>[2x]MGSSHHHHHHHSQDPAEKQKHDGRVKIGHYVLGDTLGVGTFGKVKIGEHQLTGHKVAVKILNRQKIRSLDVVGKIKREIQNLKLFRHPHIIKLYQVISTPTDFFMVMEYVSGGELFDYICKHGRVEEMEARRLFQQILSAVDYCHRHMVVHRDLKPENVLLDAHMNAKIADFGLSNMMSDGEFLRTSCGSPNYAAPEVISGRLYAGPEVDIWSCGVILYALLCGTLPFDDEHVPTLFKKIRGGVFYIPEYLNRSVATLLMHMLQVDPLKRATIKDIREHEWFKQDLPSYLFPEDPSYDANVIDDEAVKEVCEKFECTESEVMNSLYSGDPQDQLAVAYHLIIDNRRIMNQASEFYLASSPPDSFLDDHHLTRPHPERVPFLVAETPRARHTLDELNPQKSKHQGVKKAKWHLGIRSQSKPYDIMAEVYRAMKQLDFEWKVVNAYHLRVRRKNPVTGNYVKMSLQLYLVDNRSYLLDFKSIDDEVVEQRSGSSTPQRSCSAAGLHRPRSSFDSTTAESHSLSGSLTGSLTGSTLSSVSPRLGSHTMDFFEMCASLITTLAR;>MGNTSSERAALERHGGHKTPRRDSSGGTKDGDRPKILMDSPEDADLFHSEEIKAPEKEEFLAWQHDLEVNDKAPAQARPTVFRWTGGGKEVYLSGSFNNWSKLPLTRSHNNFVAILDLPEGEHQYKFFVDGQWTHDPSEPIVTSQLGTVNNIIQVKKTDFEVFDALMVDSQKCSDVSELSSSPPGPYHQEPYVCKPEERFRAPPILPPHLLQVILNKDTGISCDPALLPEPNHVMLNHLYALSIKDGVMVLSATHRYKKKYVTTLLYKPI[2x];>MADLNWETVISSDSSPAVENEHPQETP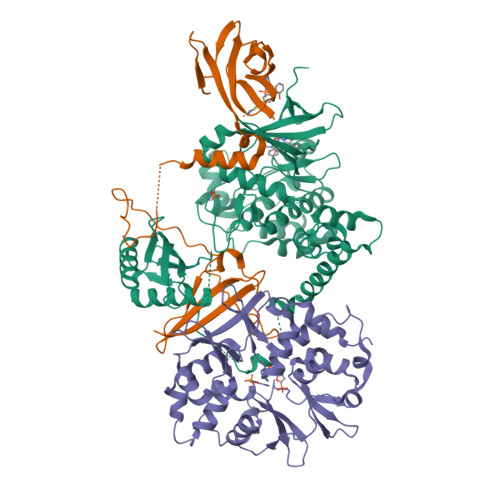ESNNSVYTSFMKSHRCYDLIPTSSKLVVFDTSLQVKKAFFALVTNGVRAAPLWDSKKQSFVGMLTITDFINILHRYYKSALVQIYELEEHKIETWREVYLQDSFKPLVCISPNASLFDAVSSLIRNKIHRLPVIDPESGNTLYILTHKRILKFLKLFITEFPKPEFMSKSLEELQIGTYANIAMVRTTTPVYVALGIFVQHRVSALPVVDEKGRVVDIYSKFDVINLAAEKTYNNLDVSVTKALQHRSHYFEGVLKCYLHETLETIINRLVEAEVHRLVVVDENDVVKGIVSLSDILQALVLTGGEKKP[2x]>MKMTFFPYELKLRHVFTVATYSRTTTPDVQVEIEYEGVTGYGEASMPPYLGETVESVMNFLKKVNLEQFSDPFQLEDILSYVDSLSPKDTAAKAAVDIALHDLVGKLLGAPWYKIWGLNKEKTPSTTFTIGIDTPDVVRAKTKECAGLFNILKVKLGRDNDKEMIETIRSVTDLPIAVDANQGWKDRQYALDMIHWLKE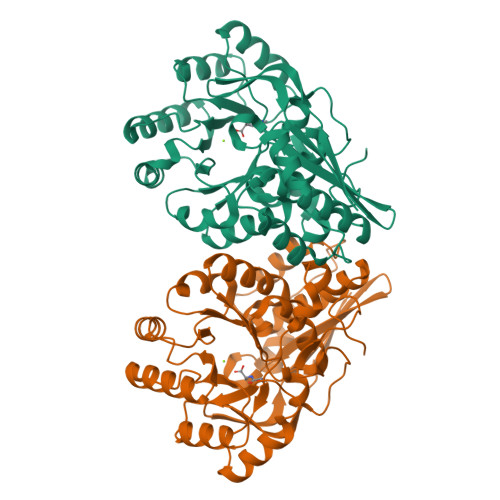KGIVMIEQPMPKEQLDDIAWVTQQSPLPVFADESLQRLGDVAALKGAFTGINIKLMKCTGMREAWKMVTLAHALGMRVMVGCMTETSCAISAASQFSPAVDFADLDGNLLISNDRFKGVEVVNGKITLNDLPGIGVMKI[2x]>[3x]GYDKDLCEWSMTADQTEVETQIEADIMNIVKRDRPEMKAEVQKQLKSGGVMQYNYVLYCDKNFNNKNIIAEVVGE

Here, we describe the structure and function of gp61.3 and show that gp61.3 inhibits the lysozyme activity of gp5 but not that of T4L. In 2002, we determined the crystal structure of gp5 that showed that gp5 consists of three domains: an N-terminal OB-fold (Oligonucleotide/Oligosaccharide-Binding fold, gp5OB-fold, residues 1–129), a lysozyme domain (gp5Lys, residues 174–339), and a needle-like C-terminal β-helical domain (gp5β, residues 389–575). We hypothesized that the mature form of Spackle/gp61.3 (residues 23–97) functions in the periplasm to selectively inhibit the activity of gp5, possibly by direct interaction. Combining all our results with previous work on gene sp and 5 mutants, we propose that the main function of the Spackle protein gp61.3 is to inhibit “free” copies of gp5 that are not incorporated into the virion during T4 particle assembly and thus can escape into the periplasm.

The structure of gp61.3 was determined by a single wavelength anomalous diffraction technique using a Se-methionine substituted protein. A 1.6 Å resolution crystal structure shows that gp61.3 is a fully α-helical globular protein. It contains 5 α-helices: helix 1 (26–34), helix 2 (37–55), helix 3 (57–70), helix 4 (73–75) and helix 5 (87–95) that are connected by short loop linkers. There are three gp61.3 monomers in the crystallographic asymmetric unit. Barring different rotamers, their structures are nearly identical. In two of the three gp61.3 molecules contained in the crystallographic asymmetric unit, a calcium ion is coordinated by several water molecules and the main chain hydroxyl groups of residues Val94 and Glu97. The thiol groups of two cysteine residues Cys29 and Cys81 are close in space, but not close enough to form a proper disulfide bond. The distance between the sulfur peaks in the electron density is 2.43 ± 0.06Å when averaged over the three molecules contained in the asymmetric unit. As a global average of billions of molecules comprising the crystal, the crystallographic electron density most likely depicts a superposition of the conformation with a disulfide bond (which has a length of 2.05 Å) and a vast number of conformations in which the thiol groups are greater than the Van der Waals distance away from each other. Hence, even though gp61.3 is a very small protein, it appears to possess a novel and possibly unique fold.>MIELSIDEKYEAEVKKSEIDHHKPTAGAMLSHVLSNIFYEKISLMQAGLYAKSANYRIKFREIALKEDEWFYLISEQLLDENELVPTTLDEFVSNHKFIENDPKAKYWTDEALIENFINDFQNQNLFIGRAIKLAQKEEKFSLELAIRKLYGYNLSIIPYFAGELGKTIGE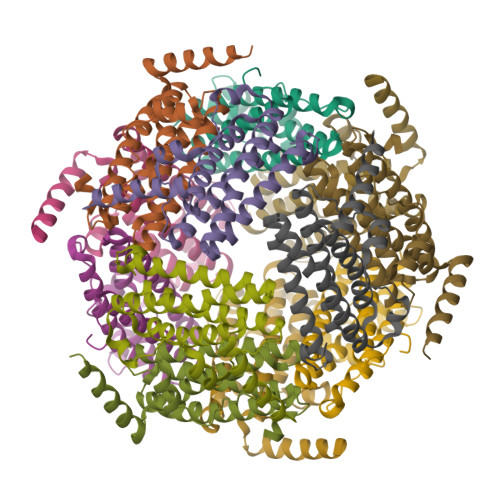FIEEEDED[4x]> GSHMASPNGQTKPLPALKLALEYIVPCMNKHGICVVDDFLGKET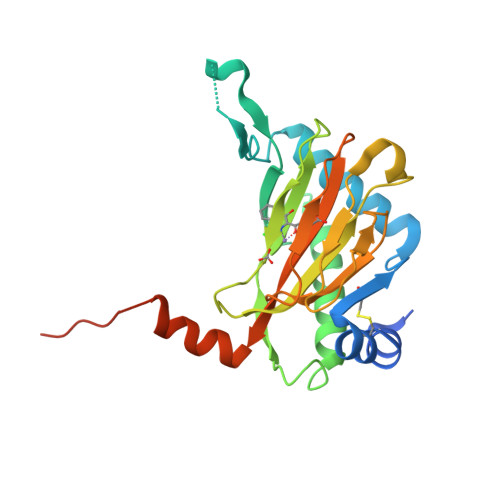GQQIGDEVRALHDTGKFTDGQLVSQKSDSSKDIRGDKITWIEGKEPGCETIGLLMSSMDDLIRHCNGKLGSYKINERTKAMVACYPGNGTGYVRHVDNPNGDGRCVTCIYYLNKDWDAKVSGGILRIFPEGKAQFADIEPKFDRLLFFWSDRRNPHEVQPAYATRYAITVWYFDADERARAKVKYLTGEKGVRVELNKPSDSVGKDVF> MRGSHHHHHHGSDETGKELVLALYDYQEKSPREVTMKKGDILTLLNSTNK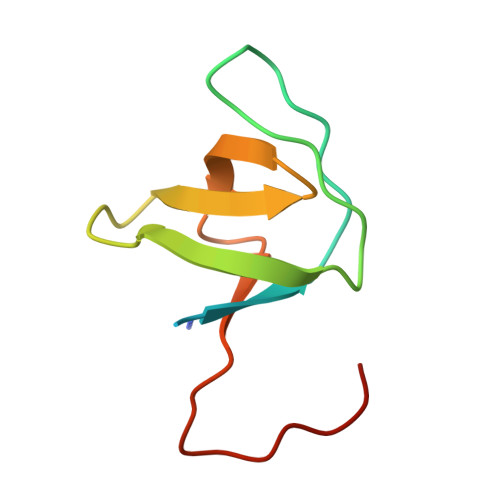DWWKVEVNDRQGFVPAAYVKKLAAAWSHPQFEK> AEPPLVFEPVTLESLRQEAGFQAVGAAQIAELDTLRAAHAAERTSVQKTQNAAIDKLIK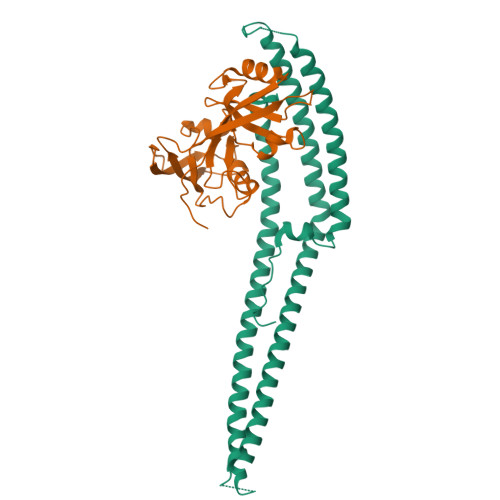GKSKDDIRNDANIKNSINDQTKQWTDMIARHRKEEWDMLRQHVQDSQDAMKALMLTVQAAQIKQLEDRHARDIKDLNAKQAKMSADTAKEVQNDKTLKTKNEKDRRLREKRQNNVKRFMEEKKQIGVKQGRAMEKLKLAHSKQIEEFSTDVQKLMDMYKIEEEAYKTQGKTEFYA;> ATAEIKPNKKILIELKVEKKPMGVIVCGGKNNHVTTGCVITHVYPEGQVAADKRLKIFDHICDINGTPIHVGSMTTLKVHQLFHTTYEKAVTLTVFRADPPELEKFNVDLMKKAGKELGLSLSPNEIGCTIADLIQGQYPEIDSKLQRGDIITKFNGDALEGLPFQVCYALFKGANGKVSMEVTRPKPTLRTEA2-[3-(dimethylamino)propyl]-1,2,3,4-tetrahydroisoquinolin-8-amine 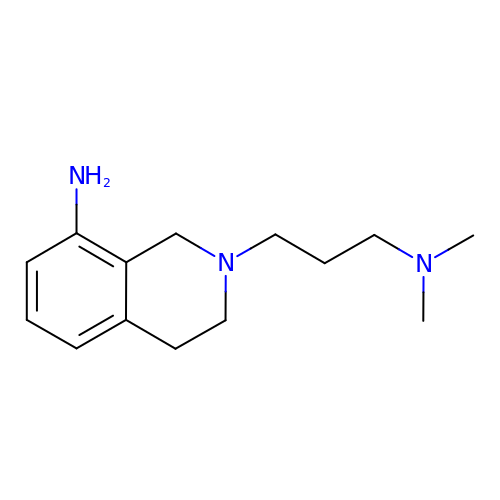| C14 H23 N3 | HWRKGGXCPROGGI-UHFFFAOYSA-N>CGATATATC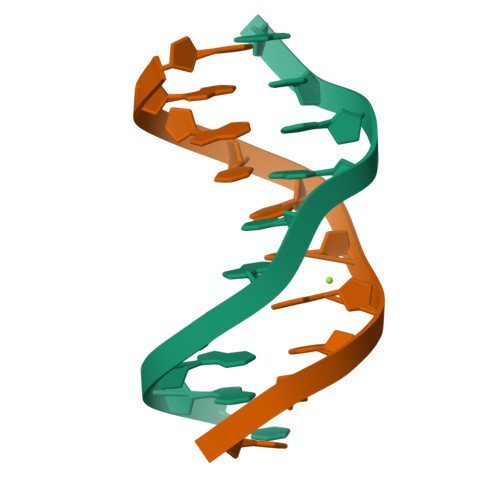G[2x]> DDVPPRIARAMENEEYWDFDIFELEAATHNRPLIYLGLKMFARFGICEFLHCSESTLRSWLQIIEANYHSSNPYHNSTHSADVLHATAYFLSKERIKETLDPIDEVAALIAATIHDVDHPGRTNSFLCNAGSELAILYNDTAVLESHHAALAFQLTTGDDKCNIFKNMERNDYRTLRQGIIDMVLATEMTKHFEHVNKFVNSINKPLATLEENGETDKNQEVIN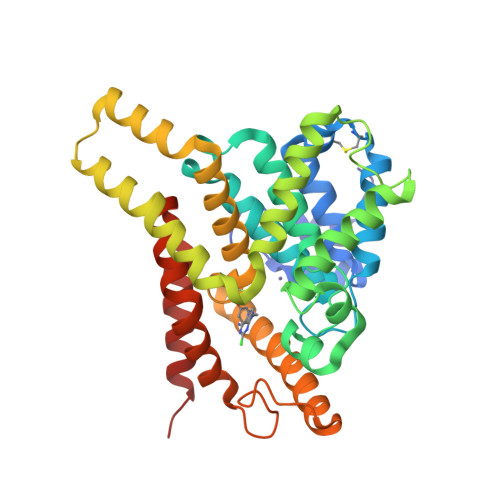TMLRTPENRTLIKRMLIKCADVSNPCRPLQYCIEWAARISEEYFSQTDEEKQQGLPVVMPVFDRNTCSIPKSQISFIDYFITDMFDAWDAFVDLPDLMQHLDNNFKYWKGLDEM>GSMPKPINVRVTTMDAELEFAIQPNTTGKQLFDQVVKTVGLREVWFFGLQYVDSKGYSTWLKLNKKVTQQDVKKENPLQFKFRAKFFPEDVSEELIQEITQRLFFLQVKEAILNDEIYCPPETAVLLASYAVQAKYGDYNKEIHKPGYLANDRLLPQRVLEQHKLTKEQWEERIQNWHEEHRGMLREDSMMEYLKIAQDLEMYGVNYFEIKNKKGTELWLGVDALGLNIYEHDDKLTPKIGFPWSEIRNISFNDKKFVIKPIDKKAPDFVFYA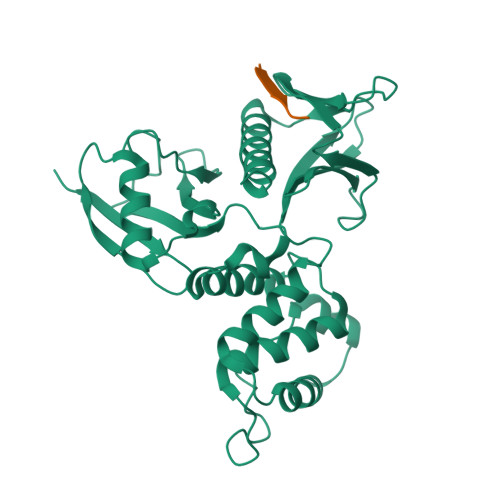PRLRINKRILALCMGNHELYMRRRKPDTIEVQQMKAQAR[3x];>[3x]GRSESQMDITDINAPKPKKKQR>[2x]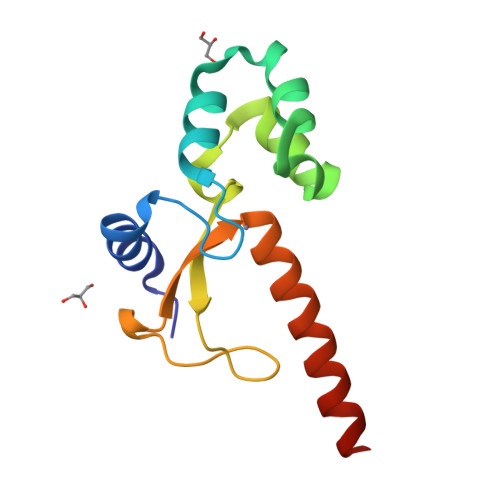SMSNNSYLRAKVFETEHGVCQLCNVNAQELFLRLRDAPKSQRKNLLYATWTSKLPLEQLNEMIRNPGEGHFWQVDHIKPVYGGGGQCSLDNLQTLCTVCHKERTARQAKERSQVRRQSLASK> EFIEIVERSNYMGNPWTEYMAKYDIEEVHGSGIRVDLGEDAEVAGTQYRLPSGKCPVFGKGIIIENSKTTFLKPVATGNQDLKDGGFAFPPTNPLISPMTLNGMRDFYKNNEYVKNLDELTLCSRHAGNMNPDNDKNSNYKYPAVYDYNDKKCHILYIAAQENNGPRYCNKDQSKRNSMFCFRPAKDKLFENYVYLSKNVVDNWEEVCPRKNLENAKFGLWVDGNCEDIPHVNEFSANDLFECNKLVFELSASDQPKQYEQHLTDYEKIKEGFKNKNADMIKSAFLPTGAFKADRYKSHGKGYNWGNYNRETQKCEIFNVKPTCLINDKSYIATTALSHPIEVEHNFPGLEQKLISEEDLNSAVDHHHHHH;> MDISQHATDIGMGPATSCYTSTIPPPKQVCIQQAVKATL

Two of these, Apical Membrane Antigen 1 (AMA1) and the Rhoptry Neck (RON) complex comprising RON2, RON4 and RON5, play a crucial role at the MJ.. In this invasion model, AMA1 and the RON complex then bind together linking the merozoite and erythrocyte membranes to form an essential structural component that maintains the MJ ring. The receptor-binding site on P. falciparum and T. gondii AMA1 (PfAMA1 and TgAMA1, respectively) comprises a region on Domain 1 of the ectoplasmic domain termed the hydrophobic groove and a region immediately adjacent that becomes exposed when the mobile Domain 2 (D2) loop (residues Ser347-His393) is displaced by the incoming ligand. We have determined the crystal structure of AMA1 from P. vivax (PvAMA1) in complex with a 39-residue peptide corresponding to the extracellular region of RON2 from P. vivax (PvRON2sp1) and, in addition, the structure of the cross-reaction complex formed between PvRON2sp1 and PfAMA1.

The heterocomplex PfAMA1-PvRON2sp1 was crystallized using recombinant PfAMA1, comprising domains D1 and D2 only, from strain FVO. The PfAMA1(FVO) polypeptide chain was traced from Arg102 to Pro442 with gaps Gly259-Arg261, Lys265-Ser268, Tyr353-Asp388 (the D2 loop); 33 of the 39 residues of the PvRON2sp1 peptide were traced from Ser2037 to Lys2069. As with the homocomplex, the bound peptide in the PfAMA1(FVO)-PvRON2sp1 heterocomplex adopts a boomerang shape. A disulphide-bridged β-hairpin formed by the central segment between the two cysteine residues constitutes one wing, and the flanking N- and C-terminal segments form the other wing. The buried surface at the PfAMA1(FVO)-PvRON2sp1 interface of the heterocomplex is 3115 Å2, larger than that of the P. vivax homocomplex. The structural differences between PfAMA1(FVO) of the heterocomplex and apo PfAMA1(3D7) are, as with the PvAMA1-PvRON2sp1 complex, largely confined to some of the loop segments that contact the ligand. The loop 172–176, which is disordered in the apo PfAMA1(3D7), could be completely traced in the heterocomplex, revealing a conformation closely matching that found in the PfAMA1 homocomplex. The loop 226–233 is displaced by more than 5 Å upon forming the complex and is essentially identical in conformation to this segment in the PfAMA1-PfRON2sp1 homocomplex. The loop 264–274, which is disordered in apo PfAMA1, contacts the N-terminal region of PvRON2sp1 but could only be partially traced. By contrast, Thr2055 (PvRON2sp1) in the heterocomplex is much closer to Arg2041 (PfRON2sp1) in the P. falciparum homocomplex as the Cα positions differ by only 0.6 Å, clearly illustrating that the P. vivax ligand partially adapts to the PfAMA1 binding site.>WSHPQFEKDEEKIDCYPDENGASAENCTARGCIWEASNSSGVPFCYFVNDLYSVSDVQYNSHGATADISLKSSVYANAFPSTPVNPLRLDVTYHKNEMLQFKIYDPNKNRYEVPVPLNIPSMPSSTPEGQLYDVLIKKNPFGIEIRRKSTGTIIWDSQLLGFTFSDMFIRISTRLPSKYLYGFGETEHRSYRRDLEWHTWGMFSRDQPPGYKKNSYGVHPYYMGLEEDGSAHGVLLLNSNAMDVTFQPLPALTYRTTGGVLDFYVFLGPTPELVTQQYTELIGRPVMVPYWSLGFQLCRYGYQNDSEIASLYDEMVAAQIPYDVQYSDIDYMERQLDFTLSPKFAGFPALINRMKADGMRVILILDPAISGNETQPYPAFTRGVEDDVFIKYPNDGDIVWGKVWPDFPDVVVNGSLDWDSQVELYRAYVAFPDFFRNSTAKWWKREIEELYNNPQNPERSLKFDGMWIDMNEPSSFVNGAVSPGCRDASLNHPPYMPHLESRDRGLSSKTLCMESQQILPDGSLVQHYNVHNLYGWSQTRPTYEAVQEVTGQRGVVITRSTFPSSGRWAGHWLGDNTAAWDQLKKSIIGMMEFSLFGISYTGADICGFFQDAEYEMCVRWMQLGAFYPFSRN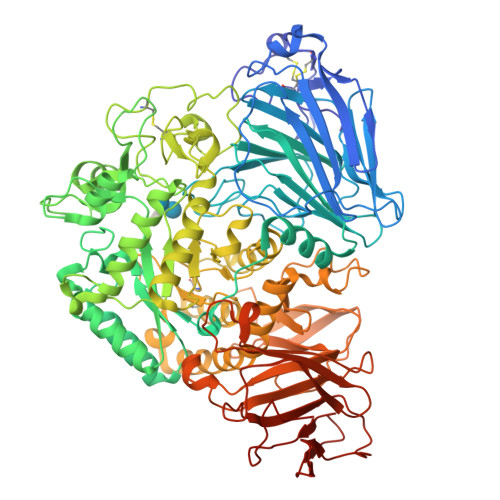HNTIGTRRQDPVSWDVAFVNISRTVLQTRYTLLPYLYTLMHKAHTEGVTVVRPLLHEFVSDQVTWDIDSQFLLGPAFLVSPVLERNARNVTAYFPRARWYDYYTGVDINARGEWKTLPAPLDHINLHVRGGYILPWQEPALNTHLSRQKFMGFKIALDDEGTAGGWLFWDDGQSIDTYGKGLYYLASFSASQNTMQSHIIFNNYITGTNPLKLGYIEIWGVGSVPVTSVSISVSGMVITPSFNNDPTTQVLSIDVTDRNISLHNFTSLTWHHHHHH[2x]> GGCGAAGAACCGGGGAGCC

k-turns are highly abundant structural motifs in RNA that generate a tight kink in the axis of RNA, mediating tertiary contacts and serving as protein binding sites. k-turns play an important structural role in a number of key cellular RNA-protein complexes, including the box C/D snoRNP, where they bind the L7Ae (in archaea) or 15.5k protein (in eukaryotes) as the first stage of assembly. Sheared G:A base pairs are frequently found in key helical junctions in RNA structure, and most notably within the core of kink turns (k-turns) as tandem G:A, A:G base pairs. We have synthesized a series of variants of the standard k-turn Kt-7 from Haloarcula marismortui in which adenine has been substituted by N6-methyladenine. We have determined the crystal structure of one of these species both free and protein-bound, showing the environment of the methyl group and the way the modification is accommodated into the k-turn structure.

By contrast, when N6-methyladenine was substituted at the A2b position the resulting Kt-7 variant underwent Mg2+-induced folding. Compared to unmodified Kt-7 the maximum EFRET value was slightly lower at 0.43, and the [Mg2+]1/2 = 275 µM, a four-fold higher concentration than required by unmodified Kt-7. Given that the N6-methyladenine 2b Kt-7 underwent folding on addition of Mg2+ ions, we investigated the structure using X-ray crystallography. Crystals of self-complementary RNA containing two Kt-7 k-turns were obtained with and without bound AfL7Ae, at resolutions of 1.99 and 2.09 Å respectively. The structure of the k-turn containing N6-methyladenine 2b is closely similar in the L7Ae bound and protein free states, superimposing with an all-atom RMSD of 0.52 Å. The resolution of the protein-free N6-methyladenine 2b Kt-7 is a little lower, and thus the position of the methyl group less well defined. Methyl groups in the syn position of N6 at either A2b or A3b are located in the minor groove, projecting out into the solvent although relatively close to the backbone of the opposite strand.> MGSSHHHHHHSQDPNSMAEDADMRNELEEMQRRADQLADESLESTRRMLQLVEESKDAGIRTLVMLDEQGEQLERIEEGMD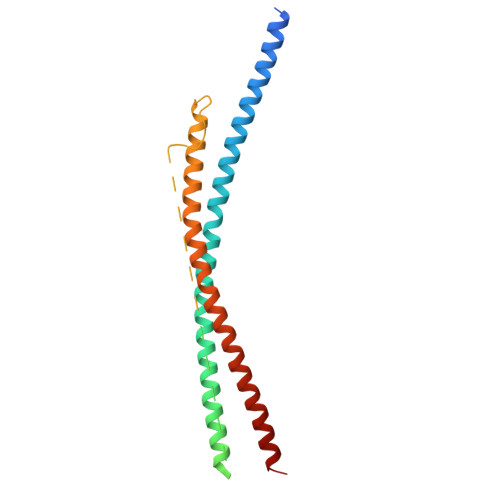QINKDMKEAEKNLTDLGKFAGLAVAPANKLKSSDAYKKAWGNNQDGVVASQPARVVDEREQMAISGGFIRRVTNDARENEMDENLEQVSGIIGNLRHMALDMGNEIDTQNRQIDRIMEKADSNKTRIDEANQRATKMLGSG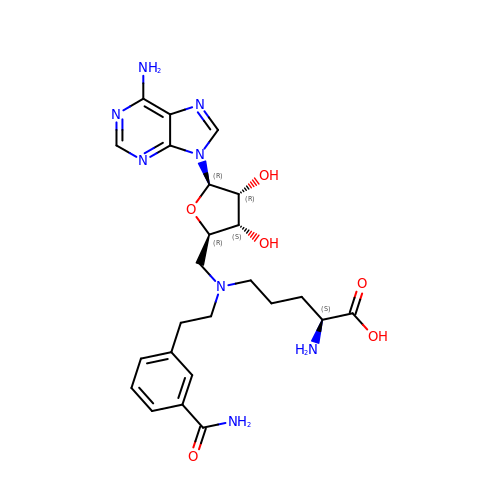(2~{S})-5-[2-(3-aminocarbonylphenyl)ethyl-[[(2~{R},3~{S},4~{R},5~{R})-5-(6-aminopurin-9-yl)-3,4-bis(oxidanyl)oxolan-2-yl]methyl]amino]-2-azanyl-pentanoic acid | C24 H32 N8 O6 | HSCPXDPGPWYINM-NMNPZVDOSA-N~{N}-(4-methoxyphenyl)-7~{H}-pyrrolo[2,3-d]pyrimidin-4-amine 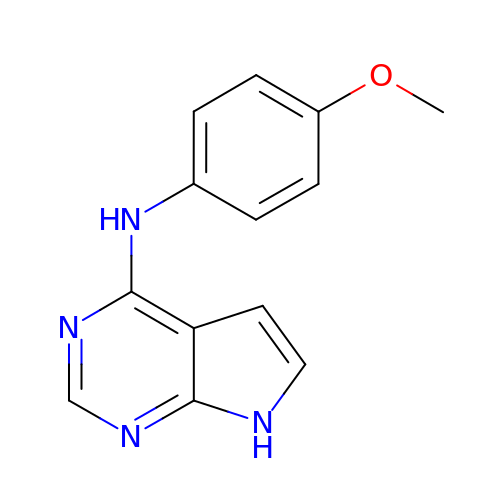| C13 H12 N4 O | DJHHJFCJDPLIQB-UHFFFAOYSA-N>NAVCRGPGDKPTQNIQLFNGRYAIINNSTAYPSRNSISELKVPRDFVPSPGTFHGCSRFPSYSNHYGLWCYSHTVSNDTCDGSNPSVQILSVGKLITGDNGQPEHKTLYTQQLSQTDRLYHCSVTMTTLGCYILCSKPRVNETQDYETIGIEPMIIGMLGLDGVYTDLGNPVGISDNSLYAMYPGPGGGVMYKDFLVFPLHGGVRFSEASKMLGKNITFRGFPPSDTCTEHEKSLTQEPANMLTSPYYGEVLVLDFLYVCTLLDNIPGECSIQLIPPDNMTMGSESKLYKLNNSLLLYKRSSSWWPYTEVYQLSLRVSKNSMKVRESVRLNITSTTRPGVEGCNINKVCPKVCVTGVFQAPGIIRKALSPKESNEDLLFFQAWTSDSIARQGPLISLCRADSCVLTIPLGNSDVFIGYTDSFCLSDRDNEKIYCVALLELDNMPYSEMTIRSFLYLIKGTETSQVAPA[2x]

Sosuga virus (SosV), from the genus Pararubulavirus, family Paramyxoviridae, is a prominent example as it has been implicated to be responsible for severe disease in an infected patient. The specific interaction between a paramyxovirus receptor-binding protein (RBP) and host-cell surface receptor during host-cell entry is a primary determinant of cellular and species tropism. As type II integral membrane proteins, paramyxoviral RBPs consist of an N-terminal cytoplasmic region, transmembrane domain, stalk region, and C-terminal six-bladed β-propeller receptor-binding domain. Here, through analysis of the RBP from SosV, an emerging member of the Pararubulavirus genus associated with human infection, we provide an integrated structural and functional rationale for how pararubulaviruses undergo sialic acid-independent host-cell entry and egress.

A soluble construct of SosV-RBP was engineered to include a portion of the N-terminal stalk region (residues 125−157) and the receptor binding β-propeller domain (residues 158−582). Residues ranging from 158 to 582 correspond to the canonical six-bladed β-propeller of the paramyxoviral attachment glycoprotein, with each blade (β1 to β6) composed of four antiparallel β-strands. Electron density corresponding to N-acetylglucosamine moieties were observed at all predicted sequons (Asn201, Asn265, Asn340, Asn403, Asn416, and Asn455), suggestive that these sites may be occupied on the native virion. Overlay analysis reveals that SosV-RBP shares the greatest level of structural conservation with orthoavula-, orthorubula-, and respirovirus HN RBPs (1.7−2.1 Å RMSD upon superposition of equivalent Cα atoms), when compared with protein-binding morbilliviral H RBPs (3.1 Å RMSD upon overlay with measles virus RBP; MV-RBP) and henipaviral G RBPs (2.2−2.3 Å RMSD). Two molecules of SosV-RBP were observed in the asymmetric unit of the crystal and form a putative homodimer through the interaction of the first (β1) and sixth (β6) blades of the β-propeller. Additionally, the angle of association between SosV-RBP protomers (31°) is substantially less than that observed in NDV-RBP, PIV3-RBP, PIV5-RBP, and MuV-RBP (average of 57°) structures. Indeed, while the glycoprotein presents some features that are conserved with paramyxoviral RBPs with known HN functionality, including a conserved cation binding site and residues that would contribute to recognition of the glycerol moeity of sialic acid, the overall configuration of the putative active site is incompatible with known modes of sialic acid recognition. First, we observe that SosV-RBP hexapeptide residues Leu243SosV-RBP and His245SosV-RBP impede into the region where the O4 of sialic acid is positioned in other paramyxovirus RBP−sialic acid complex structures.> XM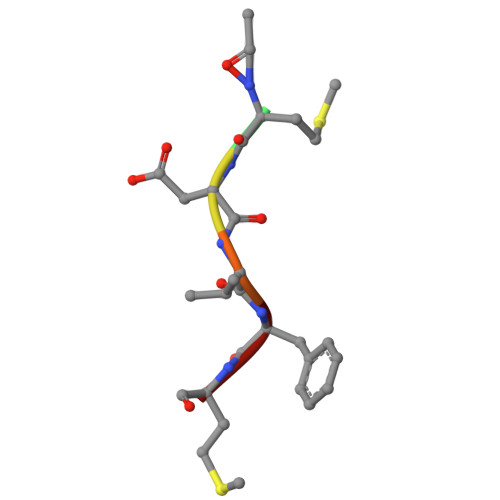DVFM>[2x]MVSKIIDIKTSIIK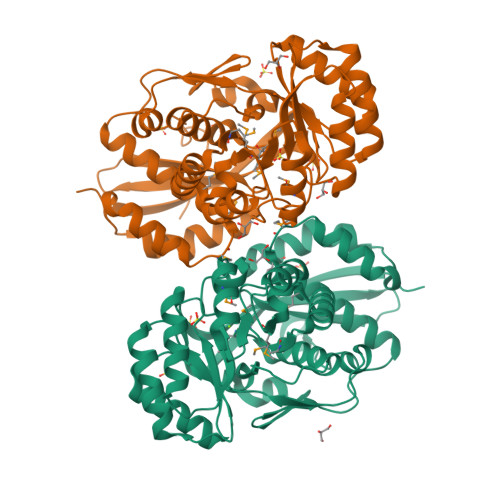IPLKRTFITAVRSTNHIDSLAVELTLDNGVKGYGVAPATTAITGDTLQGMQYIIREIFAPVILGSDLSDYKQTLELAFKKVMFNSAAKMAIDLAYHDLLAKEQDISVAKLLGAKANSIVTDVSISCGNVAETIQNIQNGVEANFTAIKVKTGADFNRDIQLLKALDNEFSKNIKFRFDANQGWNLAQTKQFIEEINKYSLNVEIIEQPVKYYDIKAMAEITKFSNIPVVADESVFDAKDAERVIDEQACNMINIKLAKTGGILEAQKIKKLADSAGISCMVGCMMESPAGILATASFALAEDITVADLDPLDWVAKDLYSDYITFNEPNIILKDNLKGFGFNLAENLYFQSHHHHHHWSHPQFEK> MFERIDYYAGDPILGLVEKFAADNNPDKVNLGIGIYYDESGVMPVL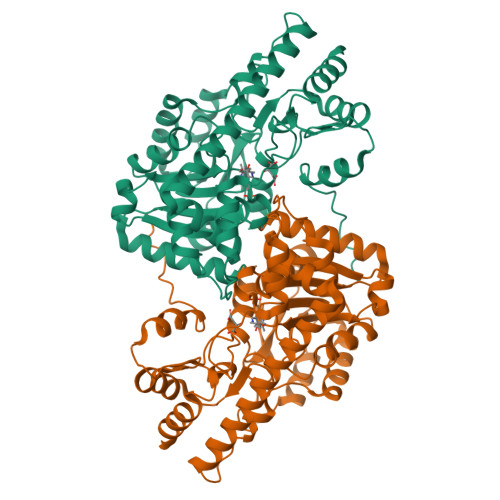DCVKIAEQRIADPISPRPYLPMAGLPGHRKGCQELLFGKDAPVLKDGLVATIATIGGSGALKVGAEFIHEWFPQSKCYVSDPTWGNHIAIFEGCDIEVGKYPYYDTATGGIKFDEMIAFFETLNKDDVLLLHPCCHNPTGVDLTREQWDTVLNVIQERELIPFMDIAYQGFGEDMDSDAYAIRKAVDMGLPLFVSNSFSKNLSLYGERVGGLSVVCPTVDETERVFGQLNSTVRRIYSSPPSHGGRVVDIVMNDAALHEQWVGEVYAMRDRIKSMRTKLKSVLEAKISGRNFDYLTAQNGMFSFTGLTPEQVERLQSEFGIYMISNSRMCVAGLNSSNIDYVANAMVDVLKD>[2x]MAAGESMAQRMVWVDLEMTGLDIEKDQIIEMACLITDSDLNILAEGPNLIIKQPDELLDSMSDWCKEHHGKSGLTKAVKESTITLQQAEYEFLSFVRQQTPPGLCP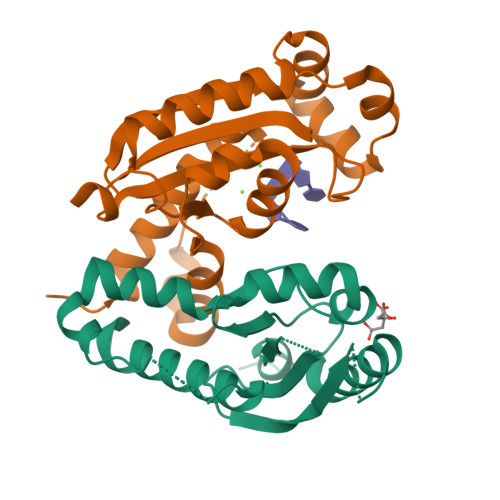LAGNSVHEDKKFLDKYMPQFMKHLHYRIIDVSTVKELCRRWYPEEYEFAPKKAASHRALDAISESIKELQFYRNNIFKKK> MEHVAFGSEDIENTLAKMDDGQLDGLAFGAIQLDGDGNILQYNAAEGDITGRDPKQVIGKNFFKDVAPCTDSPEFYGKFKEGVASGNLNTMFEYTFDYQMTPTKVKVHMKKALSGDSYWVFVKRV

In these experiments, bacterial proteins with different functions were investigated. Microcrystals of photoactive yellow protein (PYP), a blue-light photoreceptor from Halorhodospira halophila, were used to explore the capability of microsecond X-ray pulses. A nitrite-reducing enzyme, cytochrome c nitrite reductase (ccNiR) from Shewanella oneidensis, was exploited to investigate potential secondary radiation damage, caused by 90 µs pulses, at heme centers. Finally, a first TR-SSX experiment was performed on the photosensory core module (PCM) of a bacterial phytochrome from the nonphotosynthetic myxobacterium Stigmatella aurantiaca.

PYP is a small protein (14 kDa, 125 amino acids) that covalently binds p-coumaric acid (pCA) to a conserved cysteine residue via a thioester bond. We used both a fixed target and a tape drive to collect SSX data from PYP microcrystals on beamline ID29. The PYPPEG crystals belonged to space group P65. The PYPPEG crystals diffracted to higher resolution than the PYPMal crystals. PYP in space group P65 only forms four contacts between symmetry-related copies within 5 Å, while in space group P63 eight contacts are formed. Despite the denser packing of the P63 crystals, the crystals grown from PEG diffract to better resolution. Microcrystals suspended in viscous PEG are best used with fixed targets and tape drives, both of which were used in this study. The highly diffracting PYPPEG crystals were used for calibration and detector geometry refinement and for optimizing the key parameters for data collection from other proteins.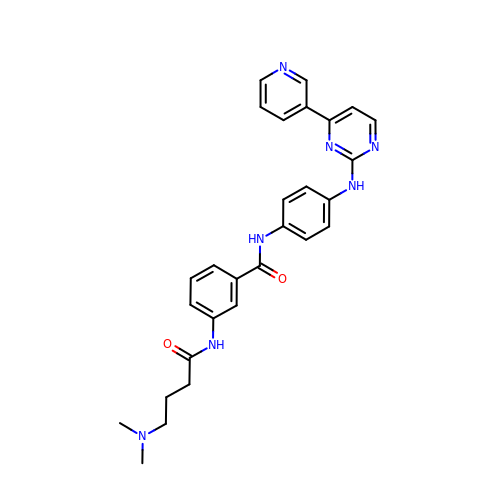3-{[4-(dimethylamino)butanoyl]amino}-N-(4-{[4-(pyridin-3-yl)pyrimidin-2-yl]amino}phenyl)benzamide | C28 H29 N7 O2 | QHAGMZSIDYTUPB-UHFFFAOYSA-N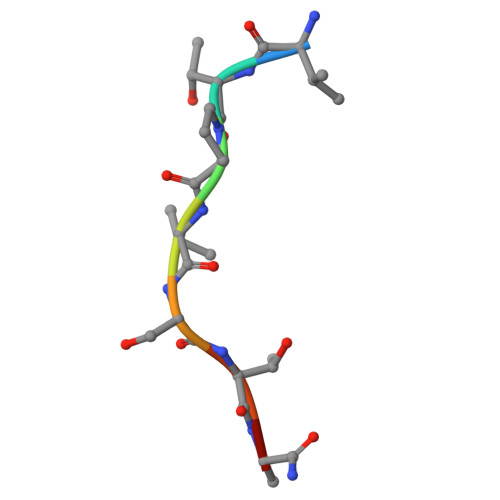> VTPVSTAA> GSHMVPAALPQLTPTLVSLLEVIEPEVLYAGYDSSVPDSAWRIMTTLNMLGGRQVIAAVKWAKAIPGFRNLHLDDQMTLLQYSWMFLMVFALGWRSYRQASGNLLCFAPDLIINEQRMTLPCMYDQCKHMLFISTELQRLQVSYEEYLCMKTLLLLSSVPKEGLKSQELFDEIRMTYIKELGKAIAKRGGNSSQNWQRFYQLTKLLDSMHDVVENLLSYCFQTFLDKSMSIEFPEMLAE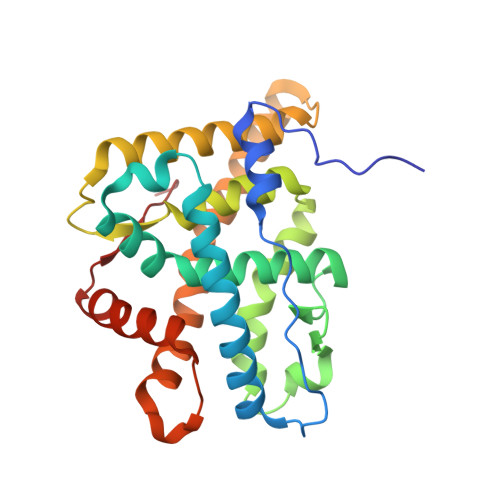IITNQIPKYSNGNIKKLLFHQK>[2x]SLLNVPAGKDLPEDIYVVIEIPANADPIKYE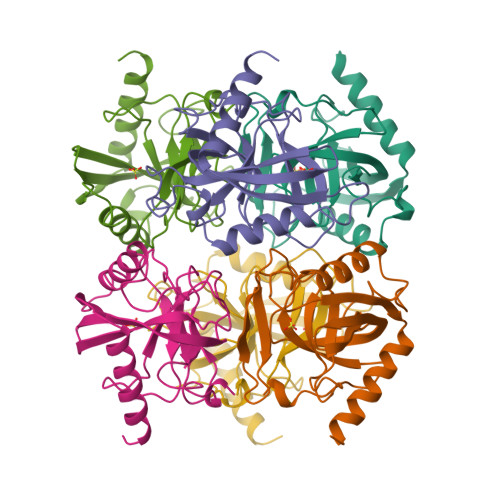IDKESGALFVDRFMSTAMFYPCNYGYINHTLSLDGDPVDVLVPTPYPLQPGSVIRCRPVGVLKMTDEAGEDAKLVAVPHSKLSKEYDHIKDVNDLPELLKAQIAHFFEHYKDLEKGKWVKVEGWENAEAAKAEIVASFERAKNK> GAGCAGACCAGA;> CGGTACTCA;> TCTCCG;> TCTGAGTAGGTCTGC

In this work, we exhaustively probe the ability of all 36 immobile HJ sequences to form DNA crystals in two different designed systems. Three separate self-assembling DNA crystal systems are described in this report: the “4 × 5” and “4 × 6” designs (collectively referred to as the 4 × N systems), and a third construct with a “scrambled” sequence variant of the 4 × 6 lattices. Self-assembly was mediated by three constituent oligonucleotides: (S1) containing four sequence repeats of either 5 or 6 bases; (S2) composed of 21 bases containing complementary regions to both (S1); and (S3) which forms the second junction crossover. The HJ serves as the fundamental component at the core of each unit, and the ultimate assembly of the full lattice is facilitated by the complementary 2-base sticky ends that tail each duplex.

In parallel, we employed the previously reported J1 4 × 6 system (3.05 Å), with P32 symmetry. Seventeen of the 36 junctions successfully crystallized, a 47% success rate. Unlike the 4 × 5 motif, nearly all of the 4 × 6 junction sequences had a strong preference for crystallization in buffers containing ≥2.0 M salts (e.g., LiCl, Li2SO4, KCl, and NaCl), with the majority preferring slightly basic pH conditions in cacodylic acid. The average cell constants for the P32 crystals were a = b = 68.29 Å c = 55.68 Å. The average junction angles of 54.60° (σ = 1.44) and 58.37° (σ = 2.3) for the P32 and R3 symmetries, respectively, along with their preference for salts or organic solvents, were likely the major contributing factors that yielded the divergent lattices.> MWADEEPAPWDIEETPAEQAPEASAESAAPAAEAATGEKPKIKLEKIEPPHYNHHWVRPLFLNYAYYLYEYRKNYYNDVIDYLNQREKGIFREPPRAQEWAERAMRTYDEKNTDKSFKRSADMKYI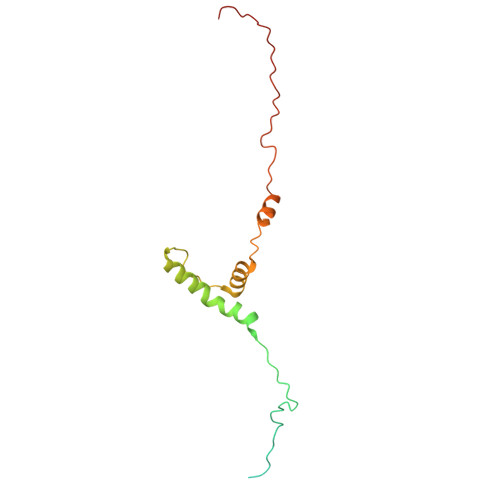INMRHEPRYYSYHTRAYYSLKYQKIL Leukotriene A4 hydrolase (LTA4H) is a zinc metalloenzyme that stands out with unique dual functionalities that include peptidase activity in addition to lipid metabolism. As an epoxide hydrolase (EH), LTA4H converts leukotriene A4 (LTA4) to leukotriene B4 (LTB4). As an aminopeptidase (AP), LTA4H hydrolyzes natural ligands such as dynorphin, enkephalin, and the tripeptide proline-glycine-proline (PGP), of which PGP has garnered significant interest. Therefore, bi-functional EH and AP activities undergird the intricate pro- and anti-inflammatory regulation, respectively, exerted by LTA4H.

As shown in the M1 metallopeptidase HEXXH-(X)18E motif, the Zn2+ ion was coordinated with H295, E296 H299, and the carboxylic acid side chain oxygen atom of E31826. Our interpretation is that the Q136 side chain maintains the catalytic water molecule interaction with E296 while simultaneously engaging in multiple hydrophobic interactions via its rotational freedom. The loss of water molecules could afford more favorable binding entropies for nonpolar ligand binding, provided steric clashes are avoided. Also, the structural data suggest that nonpolar ligands are likely necessary for enhancing the peptidase activity due to more favorable binding entropies in the active site. Hence hydrophobic interactions and steric considerations are the primary factors influencing what modified kinetics may be possible.

>IVDTCSLASPASVCRTKHLHLRCSVDFTRRTLTGTAALTVQSQEDNLRSLVLDTKDLTIEKVVINGQEVKYALGERQSYKGSPMEISLPIALSKNQEIVIEISFETSPKSSALQWLTPEQTSGKEHPYLFSQCQAIHCRAILPCQDTPSVKLTYTAEVSVPKELVALMSAIRDGETPDPEDPSRKIYKFIQKVPIPCYLIALVVGALESRQIGPRTLVWSEKEQVEKSAYEFSETESMLKIAEDLGGPYVWGQYDLLVLPPSFPYGGMENPCLTFVTPTLLAGDKSLSNVIAHEISHSWTGNLVTNKTWDHFWLNEGHTVYLERHICGRLFGEKFRHFNALGGWGELQNSVKTFGETHPFTKLVVDLTDIDPDVAYSSVPYEKGFALLFYLEQLLGGPEIFLGFLKAYVEKFSYKSITTDDWKDFLYSYFKDKVDVLNQVDWNAWLYSPGLPPIKPNYDMTLTNACIALSQRWITAKEDDLNSFNATDLKDLSSHQLNEFLAQTLQRAPLPLGHIKRMQEVYNFNAINNSEIRFRWLRLCIQSKWEDAIPLALKMATEQGRMKFTRPLFKDLAAFDKSHDQAVRTYQEHKASMHPVTAMLVGKDLKVD[3x]> MASWSHPQFEKGADDDDKVPDPTSVDSVKYSKIKGIPKLDDANDAGGKHSLECTLILTEGDSAKSLAVSGLGVIGRDRYGVFPLRGKILNVREASHKQIMENAEINNIIKIVGLQYKKSYDDAESLKTLRYGKIMIMTDQDQDGSHIKGLLINFIHHNWPSLLKHGFLEEFITPIVKASKNKQELSFYSIPEFDEWKKHIENQKAWKIKYYKGLGTSTAKEAKEYFADMERHRILFRYAGPEDDAAITLAFSKKKIDDRKEWLTNFMEDRRQRRLHGLPEQFLYGTATKHLTYNDFINKELILFSNSDNERSIPSLVDGFKPGQRKVLFTCFKRNDKREVKVAQLAGSVAEMSAYHHGEQALMMTIVNLAQNFVGSNNINLLQPIGQFGTRLHGGKDAASPRYIFTMLSTLARLLFPAVDDNLLKFLYDDNQRVEPEWYIPIIPMVLINGAEGIGTGWACKLPNYDAREIVNNVRRMLDGLDPHPMLPNYKNFKGTIQELGQNQYAVSGEIFVVDRNTVEITELPVRTWTQVYKEQVLEPMLNGTDKTPALISDYKEYHTDTTVKFVVKMTEEKLAQAEAAGLHKVFKLQTTLTCNSMVLFDHMGCLKKYETVQDILKEFFDLRLSYYGLRKEWLVGMLGAESTKLNNQARFILEKIQGKITIENRSKKDLIQMLVQRGYESDPVKAWKEAQEKAAEEDETQNQHDDSSSDSGTPSGPDFNYILNMSLWSLTKEKVEELIKQRDAKGREVNDLKRKSPSDLWKEDLAAFVEELDKVESQEREDGAPGFSSISAHHHHHHHHHH

Type IIA topoisomerases (Top2s) are essential DNA-manipulating enzymes ubiquitous in eukaryotes and bacteria. These enzymes exploit protein conformational changes driven by ATP binding and hydrolysis to direct the crossing of two DNA duplexes, leading to topological inversion of DNA crossovers. The Top2-mediated DNA topological transformation requires the temporary creation of a DNA double-strand break (DSB) on one DNA segment (the G-segment), so that another duplex strand (the T-segment) can be transported through.

We determined the structure of the binary complex formed by the DNA-binding and cleavage core of human topoisomerase 2β (hTop2βcore) and a 20-bp duplex DNA in a new crystal form, at 2.75-Å resolution, by molecular replacement. The asymmetric unit contains one protein subunit bound to a 9-bp DNA duplex, about half the length of the palindromic DNA used for the preparation of the dimeric Top2 cleavage complex. In contrast, the current structure adopts a quaternary conformation whose dimeric architecture is held solely by the interactions formed between the two C-gate regions without any direct or indirect contacts being observed between the two WHD domains. As the G-segment-binding grooves of the two monomers have moved away from each other, the continuous G-segment-binding surface that spans across the two WHD domains in the closed structure is disrupted, and a funnel-shaped trough is revealed between the two halves of the DNA-gate, effectively opening an entryway for the T-segment. This conformation may thus be taken as a crystallographic snapshot of the DNA-gate in an “open” state during the Top2 functional cycle. Similar to the structures commonly observed for the Top2 cleavage complexes with closed DNA-gate, a divalent metal ion, coordinated by the DxD di-acidic metal ion-binding motif of the TOPRIM domain near the non-scissile phosphodiester between the −1 and −2 nucleotides, was observed at the so-called “B-site” in our structure. However, rather than remaining coaxial, the helical axes of the two DNA fragments in the open form reported here are found to be offset in opposite directions by ~20°, relative to the original G-segment axis. Thus, the sliding of the two subunits against each other, plus the swinging of the two halves of DNA-gate regions away from the structural dyad of Top2, both contribute to the opening of the DNA-gate. However, as the channel’s bottom opening is narrower than the diameter of duplex DNA, further widening of this “bottleneck” region must take place for T-segment to go through.>MAHHHHHHVGTNTGGVLVITDTIIVKSGQTYDGKGIKIIAQGMGDGSQSENQKPIFKLEKGANLKNVIIGAPGCDGIHCYGDNVVENVVWEDVGEDALTVKSEGVVEVIGGSAKEAADAVFQLNAPCTFKVK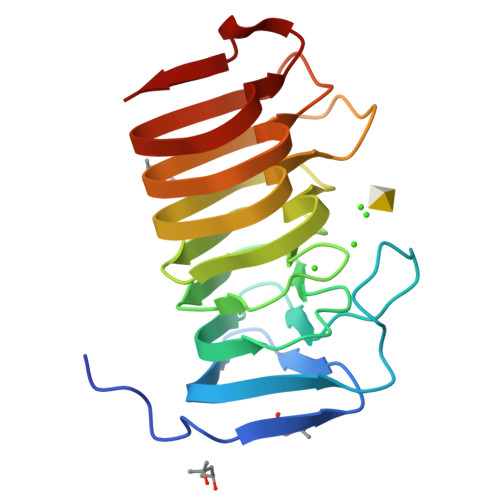NFTATNIGKLVAQNGNTTFKVVIYLEDVTLNNVKSCVAKSDSPVSELWYHNLNVNNCKTLFEFPSQSQIHQY[2x]Langerin, a C-type lectin on Langerhans cells, mediates carbohydrate-dependent uptake of pathogens in the first step of antigen presentation to the adaptive immune system. The extracellular portion of langerin contains a C-type carbohydrate recognition domain (CRD)2 that binds sugars and a neck region that mediates formation of trimers stabilized by a coiled-coil of α-helices. As in other C-type lectins, the CRD of langerin contains a primary Ca2+-dependent sugar-binding site where Ca2+ forms direct coordination bonds with two vicinal hydroxyl groups of a monosaccharide. Langerin binds to a diverse set of glycan ligands including high mannose structures, β-glucans, and fucosylated blood group antigens.

A commonly occurring single nucleotide polymorphism (SNP) in human langerin results in change of one of these lysine residues, Lys-313, to isoleucine. To determine the molecular basis for the enhanced binding of GlcNAc-terminated glycans caused by the K313I change, crystal structures of the carbohydrate recognition domains of langerin-I313, langerin-D288/I313, and wild type langerin in complex with GlcNAc, α-Me-GlcNAc, and two GlcNAc-terminated trisaccharides (GlcNAcβ1-3Galβ1-4Glcβ-CH2CH2N3 (TR54) and GlcNAcβ1-3Galβ1-4GlcNAcβ-CH2CH2N3 (TR55)), representing the terminal portions of poly N-acetyllactosamine chains that are ligands for langerin detected on the glycan array, were solved. The position of α-Me-GlcNAc bound to the CRD of langerin-I313, is analogous the position of mannose in the wild type CRD described previously. The 3- and 4-OH groups of the sugar are coordinated to the principal Ca2+ and form hydrogen bonds with Glu-293 and Asn-307 and with Asn-287 and Glu-285, respectively. However, the equatorial N-acetyl substituent at the two position of GlcNAc makes several additional secondary contacts, including water-mediated hydrogen bonds with Lys-299 and Asn-297. In addition, there are van der Waals contacts with Pro-310, which in turn interacts with Ile-313. An alternate rotamer of the Ile-313 side chain brings it into direct van der Waals contact with the N-acetyl group of the GlcNAc. One or more of these factors may explain the increased binding of the Ile-313 variant to GlcNAc. Structural analysis shows that enhanced binding to GlcNAc may result from Ile-313 packing against the N-acetyl group. Interestingly, langerin-I313 shows enhanced binding of many GlcNAc-terminated glycans, for example glycans 536, 584, 547, 177, 179, and 531, as compared with wild type langerin, which binds only weakly to these glycans.

>[4x]QVVSQGWKYFKGNFYYFSLIPKTWYSAEQFCVSRNSHLTSVTSESEQEFLYKTAGGLIYWIGLTKAGMEGDWSWVDDTPFNKVQSARFWIPGEPNNAGNNEHCGNIKAPSLQAWNDAPCDITFLFICKRPYVPSEP>MHHHHHHHHPDLGTGSENLYFQGLNSTAQGQLKSIIERVERLEVEKAEIMEQIKEVYAEAKGNGFDVKVLKKVVRIRKQDRAKRQEEDAILDLYLS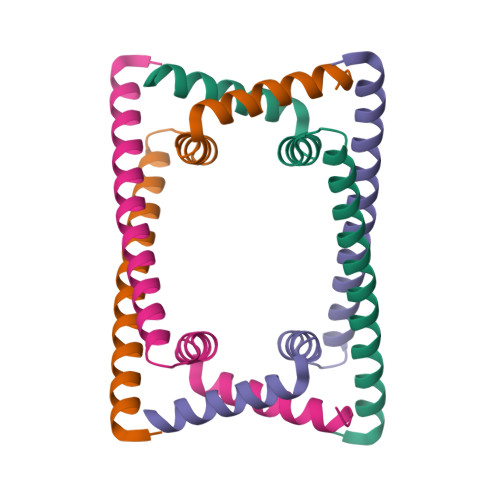AIGEI[6x]> ADSTIT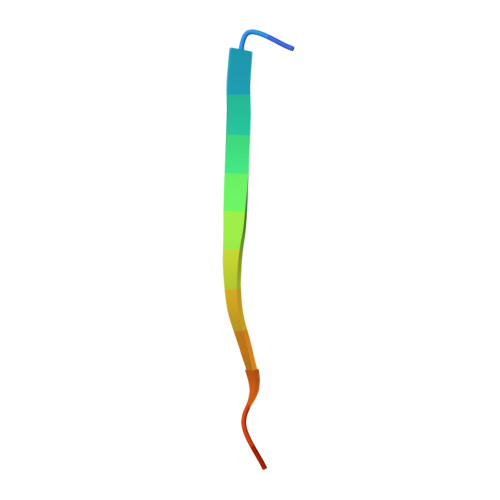IRGYVRDNG>[2x]PISPIETVPVKLKPGMDGPKVKQWPLTEEKIKALVEICTEMEKEGKISKIGPENPYNTPVFAIKKKDSTKWRKLVDFRELNKRTQDFWEVQLGIPHPAGLKKKKSVTVLDVGDAYFSVPLDEDFRKYTAFTIPSINNETPGIRYQYNVLPQGWKGSPAIFQSSMTKILEPFRKQNPDIVIYQYMDDLYVGSDLEIGQHRTKIEELRQHLLRWGLTTPDKKHQKEPPFLWMGYELHPDKWTVQPIVLPEKDSWTVNDIQKLVGKLNWASQIYPGIKVRQLCKLLRGTKALTEVIPLTEEAELELAENREILKEPVHGVYYDPSKDLIAEIQKQGQGQWTYQIYQEPFKNLKTGKYARMRGAHTNDVKQLTEAVQKITTESIVIWGKTPKFKLPIQKETWETWWTEYWQAT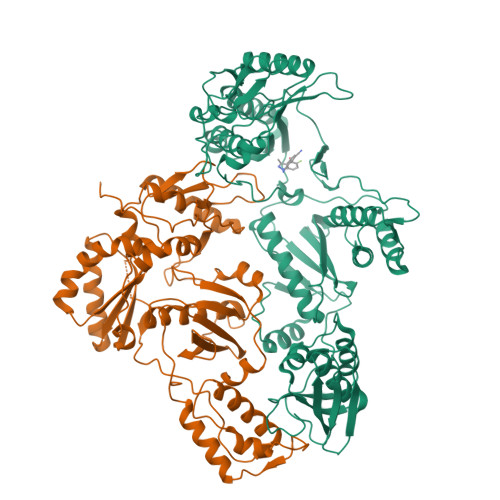WIPEWEFVNTPPLVKLWYQLEKEPIVGAETFYVDGAANRETKLGKAGYVTNRGRQKVVTLTDTTNQKTELQAIYLALQDSGLEVNIVTDSQYALGIIQAQPDQSESELVNQIIEQLIKKEKVYLAWVPAHKGIGGNEQVDKLVSAGIRKVLFLDGID D-ribitol | C5 H12 O5 | 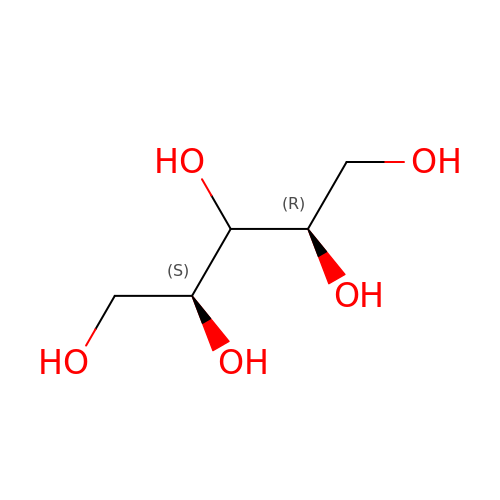HEBKCHPVOIAQTA-ZXFHETKHSA-N> GPGSMADRGLPSEAPVVTTSPAGPPSDGPMQRLLASLAGLRQPPTPTAETANGADDPAFLATAKLRAAMAAFLLSGTAIAPADARDCWRPLLEHLCALHRAHGLPETALLAENLPGLLVHRLVVALPEAPDQAFREMEVIKDTILAVTGSDTSHALDSAGLRTAAALGPVRVRQCAVEWIDRWQTVTKSCLAMSPRTSIEALGETSLKMAPVPLGQPSANLTTPAYSLLFPAPFVQEGLRFLALVSNRVTLFSAHLQRIDDATLTPLTRALFTLALVDEYLTTPERGAVVPPPLLAQFQHTVREIDPAIMIPPLEANKMVRSREEVRVSTALSRVSPRSACAPPGTLMARVRTDVAVFDPDVPFLSSSALAVFQPAVSSLLQLGEQPSAGAQQRLLALLQQTWTLIQNTNSPSVVINTLIDAGFTPSHCTHYLSALEGFLAAGVPARTPTGHGLGEVQQLFGCIALAGSNVFGLAREYGYYANYVKTFRRVQGASEHTHGRLCEAVGLSGGVLSQT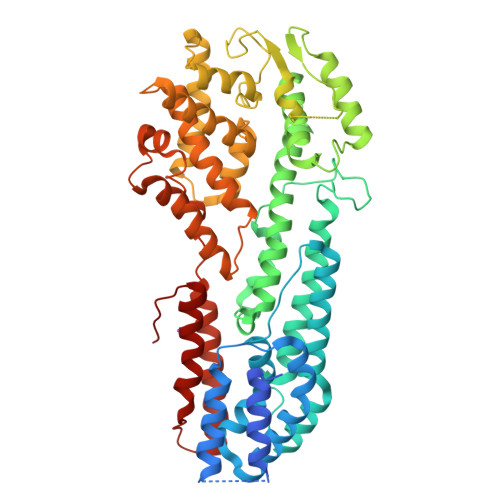LARIMGPAVPTEHLASLRRALVGEFETAERRFSSGQPSLLRETALIWIDVYGQTHWDITPTTP Here, we show that coating the cryo-EM grid surface with ssDNA, or other negatively charged polyelectrolytes, reduced sample aggregation and improved the distribution of macromolecules in holey carbon grids for cryo-EM. The samples used for testing, hexamerin, human 80S ribosome and apoferritin, exhibited undesirable properties such as protein aggregation and/or affinity for the carbon support on standard cryo-EM grids. The use of polyelectrolyte-coated grids was essential for the determination of macromolecular structures from these samples. Hexamerin, human 80S ribosome and apoferritin are soluble macromolecular complexes with a predominantly negative surface charge.

Human 80S ribosome has a molecular weight of 4.3 MDa. The first cryo-EM structure of human 80S ribosome was solved to a resolution of 3.6 Å by Bruno Klaholz’s group in 2015. The test sample of 80S ribosome at a concentration of 1.2 mg ml−1 in 25 mM HEPES pH 7.5, 125 mM KCl, 5 mM magnesium acetate, 1 mM DTT, 0.01% DDM buffer exhibited nearly complete particle aggregation on standard cryo-EM grids. Electron micrographs from these grids could not be used for cryo-EM reconstruction. The sample used in our experiments was damaged during purification and therefore exhibited aggregation during sample preparation using standard cryo-EM grids. In contrast, DNA-coated grids contained separated particles. The coating of grids with DNA was crucial for the structure determination of the 80S ribosome from our sample. The structure solved from the DNA-coated grids is identical to the previously solved ribosome structure, with a cross-correlation of 0.92 between the two cryo-EM maps. For the human 80S ribosome, which has a diameter of 25 nm, the distances were 29 ± 4 and 39 ± 9 nm, respectively.

> CGCGACCUCAGAUCAGACGUGGCGACCCGCUGAAUUUAAGCAUAUUAGUCAGCGGAGGAGAAGAAACUAACCAGGAUUCCCUCAGUAACGGCGAGUGAACAGGGAAGAGCCCAGCGCCGAAUCCCCGCCCCGCGGCGGGGCGCGGGACAUGUGGCGUACGGAAGACCCGCUCCCCGGCGCCGCUCGUGGGGGGCCCAAGUCCUUCUGAUCGAGGCCCAGCCCGUGGACGGUGUGAGGCCGGUAGCGGCCCCCGGCGCGCCGGGCCCGGGUCUUCCCGGAGUCGGGUUGCUUGGGAAUGCAGCCCAAAGCGGGUGGUAAACUCCAUCUAAGGCUAAAUACCGGCACGAGACCGAUAGUCAACAAGUACCGUAAGGGAAAGUUGAAAAGAACUUUGAAGAGAGAGUUCAAGAGGGCGUGAAACCGUUAAGAGGUAAACGGGUGGGGUCCGCGCAGUCCGCCCGGAGGAUUCAACCCGGCGGCGGGUCCGGCCGUGUCGGCGGCCCGGCGGAUCUUUCCCGCGCGGGGGACCGUCCCCCGACCGGCGACCGGCCGCCGCCGGGCGCAUUUCCACCGCGGCGGUGCGCCGCGACCGGCUCCGGGACGGCUGGGGAAGGCCCGGCGGGGAAGGUGGCUCGGGGGCCCCCGAGUGUUACAGCCCCCCCGGCAGCAGCACUCGCCGAAUCCCGGGGCCGAGGGAGCGAGACCCGUCGCCGCGCUCUCCCCCCUCCCGGCGCGCCGGGGGGGGCCGGGCCACCCCUCCCACGGCGCGACCGCUCGGGGCGGACUGUCCCCAGUGCGCCCCGGGCGGGUCGCGCCGUCGGGCCCGGGGGAGGCCACGCGCGCGUCCCCCGAAGAGGGGGACGGCGGAGCGAGCGCACGGGGUCGGCGGCGACGUCGGCUACCCACCCGACCCGUCUUGAAACACGGACCAAGGAGUCUAACACGUGCGCGAGUCGGGGGCUCGCACGAAAGCCGCCGUGGCGCAAUGAAGGUGAAGGCCGGCGCGCUCGCCGGCCGAGGUGGGAUCCCGAGGCCUCUCCAGUCCGCCGAGGGCGCACCACCGGCCCGUCUCGCCCGCCGCGCCGGGGAGGUGGAGCACGAGCGCACGUGUUAGGACCCGAAAGAUGGUGAACUAUGCCUGGGCAGGGCGAAGCCAGAGGAAACUCUGGUGGAGGUCCGUAGCGGUCCUGACGUGCAAAUCGGUCGUCCGACCUGGGUAUAGGGGCGAAAGACUAAUCGAACCAUCUAGUAGCUGGUUCCCUCCGAAGUUUCCCUCAGGAUAGCUGGCGCUCUCGCAGACCCGACGCCCGCCACGCAGUUUUAUCCGGUAAAGCGAAUGAUUAGAGGUCUUGGGGCCGAAACGAUCUCAACCUAUUCUCAAACUUUAAAUGGGUAAGAAGCCCGGCUCGCUGGCGUGGAGCCGGGCGUGGAAUGCGAGUGCCUAGUGGGCCACUUUUGGUAAGCAGAACUGGCGCUGCGGGAUGAACCGAACGCCGGGUUAAGGCGCCCGAUGCCGACGCUCAUCAGACCCCAGAAAAGGUGUUGGUUGAUAUAGACAGCAGGACGGUGGCCAUGGAAGUCGGAAUCCGCUAAGGAGUGUGUAACAACUCACCUGCCGAAUCAACUAGCCCUGAAAAUGGAUGGCGCUGGAGCGUCGGGCCCAUACCCGGCCGUCGCCGGCAGUCGAGAGUGGACGGGAGCGGCGGGCCGGAGCCCCGCGGACGCUACGCCGCGACGAGUAGGAGGGCCGCUGCGGUGAGCCUUGAAGCCUAGGGCGCGGGCCCGGGUGGAGCCGCCGCAGGUGCAGAUCUUGGUGGUAGUAGCAAAUAUUCAAACGAGAACUUUGAAGGCCGAAGUGGAGAAGGGUUCCAUGUGAACAGCAGUUGAACAUGGGUCAGUCGGUCCUGAGAGAUGGGCGAGCGCCGUUCCGAAGGGACGGGCGAUGGCCUCCGUUGCCCUCGGCCGAUCGAAAGGGAGUCGGGUUCAGAUCCCCGAAUCCGGAGUGGCGGAGAUGGGCGCCGCGAGGCGUCCAGUGCGGUAACGCGACCGAUCCCGGAGAAGCCGGCGGGAGCCCCGGGGAGAGUUCUCUUUUCUUUGUGAAGGGCAGGGCGCCCUGGAAUGGGUUCGCCCCGAGAGAGGGGCCCGUGCCUUGGAAAGCGUCGCGGUUCCGGCGGCGUCCGGUGAGCUCUCGCUGGCCCUUGAAAAUCCGGGGGAGAGGGUGUAAAUCUCGCGCCGGGCCGUACCCAUAUCCGCAGCAGGUCUCCAAGGUGAACAGCCUCUGGCAUGUUGGAACAAUGUAGGUAAGGGAAGUCGGCAAGCCGGAUCCGUAACUUCGGGAUAAGGAUUGGCUCUAAGGGCUGGGUCGGUCGCGGCCGGCGCCUAGCAGCCGACUUAGAACUGGUGCGGACCAGGGGAAUCCGACUGUUUAAUUAAAACAAAGCAUCGCGAAGGCCCGCGGCGGGUGUUGACGCGAUGUGAUUUCUGCCCAGUGCUCUGAAUGUCAAAGUGAAGAAAUUCAAUGAAGCGCGGGUAAACGGCGGGAGUAACUAUGACUCUCUUAAGGUAGCCAAAUGCCUCGUCAUCUAAUUAGUGACGCGCAUGAAUGGAUGAACGAGAUUCCCACUGUCCCUACCUACUAUCCAGCGAAACCACAGCCAAGGGAACGGGCUUGGCGGAAUCAGCGGGGAAAGAAGACCCUGUUGAGCUUGACUCUAGUCUGGCACGGUGAAGAGACAUGAGAGGUGUAGAAUAAGUGGGAGGCCCCCGGCGCCCCCCCGGUGUCCCCGCGAGGGGCCCGGGGCGGGGUCCGCCGGCCCUGCGGGCCGCCGGUGAAAUACCACUACUCUGAUCGUUUUUUCACUGACCCGGUGAGGCGGGGGGGCGAGCCCCGAGGGGCUCUCGCUUCUGGCGCCAAGCGCCCGGCCGCGCGCCGGCCGGGCGCGACCCGCUCCGGGGACAGUGCCAGGUGGGGAGUUUGACUGGGGCGGUACACCUGUCAAACGGUAACGCAGGUGUCCUAAGGCGAGCUCAGGGAGGACAGAAACCUCCCGUGGAGCAGAAGGGCAAAAGCUCGCUUGAUCUUGAUUUUCAGUACGAAUACAGACCGUGAAAGCGGGGCCUCACGAUCCUUCUGACCUUUUGGGUUUUAAGCAGGAGGUGUCAGAAAAGUUACCACAGGGAUAACUGGCUUGUGGCGGCCAAGCGUUCAUAGCGACGUCGCUUUUUGAUCCUUCGAUGUCGGCUCUUCCUAUCAUUGUGAAGCAGAAUUCACCAAGCGUUGGAUUGUUCACCCACUAAUAGGGAACGUGAGCUGGGUUUAGACCGUCGUGAGACAGGUUAGUUUUACCCUACUGAUGAUGUGUUGUUGCCAUGGUAAUCCUGCUCAGUACGAGAGGAACCGCAGGUUCAGACAUUUGGUGUAUGUGCUUGGCUGAGGAGCCAAUGGGGCGAAGCUACCAUCUGUGGGAUUAUGACUGAACGCCUCUAAGUCAGAAUCCCGCCCAGGCGGAACGAUACGGCAGCGCCGCGGAGCCUCGGUUGGCCUCGGAUAGCCGGUCCCCCGCCGGGGUCCGGUGCGGAGUGCCCUUCGUCCUGGGAAACGGGGCGCGGCCGGAGAGGCGGCCGCCCCCUCGCCCGUCACGCACCGCACGUUCGUGGGGAACCUGGCGCUAAACCAUUCGUAGACGACCUGCUUCUGGGUCGGGGUUUCGUACGUAGCAGAGCAGCUCCCUCGCUGCGAUCUAUUGAAAGUCAGCCCUCGACACAAGGGUUUGU>SNALSIPEDYQARLQPNRVEGSYPLVRMEFTGATVDAPLMSQISRKYNIDVSILSSDLDYAGGVKFGMMVAELF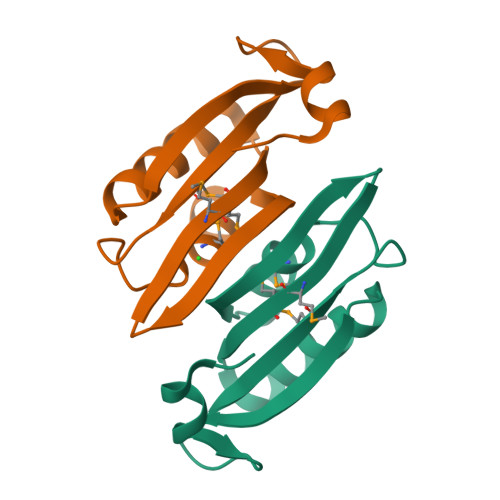GNEQDDSAAIEYLRENNVKVEVLGYVL[2x]> D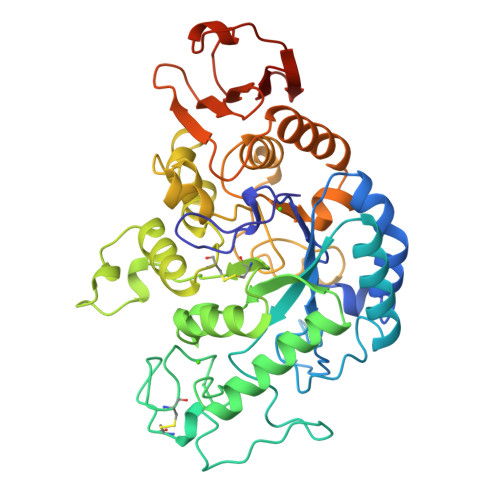QAGKSPNAVRYHGGDEIILQGFHWNVVREAPNDWYNILRQQAATIAADGFSAIWMPVPWRDFSSWSDGSKSGGGEGYFWHDFNKNGRYGSDAQLRQAASALGGAGVKVLYDVVPNHMNRGYPDKEINLPAGQGFWRNDCADPGNYPNDCDDGDRFIGGDADLNTGHPQVYGMFRDEFTNLRSQYGAGGFRFDFVRGYAPERVNSWMTDSADNSFCVGQLWKGPSEYPNWDWRNTASWQQIIKDWSDRAKCPVFDFALKERMQNGSIADWKHGLNGNPDPRWREVAVTFVDNHDTGYSPGQNGGQHHWALQDGLIRQAYAYILTSPGTPVVYWDHMYDWGYGDFIRQLIQVRRAAGVRADSAISFHSGYSGLVATVSGSQQTLVVALNSDLGNPGQVASGSFSEAVNASNGQVRVWRSGTGSGGGEPGA>SMEQLKHCNGILKELLSKKHAAYAWPFYKPVDASALGLHDYHDIIKHPMDLSTVKRKMENRDYRDAQEFAADVRLMFSNCYKYNPPDHDVVAMAR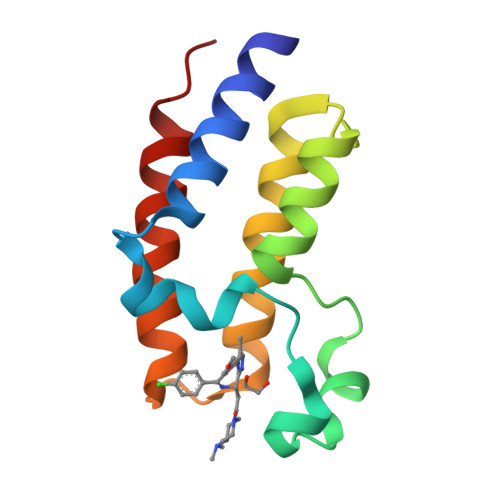KLQDVFEFRYAKMPD[2x]>ESQPSVFQCKKCFQIVGDSNAWVISHREYLSFTLSDAVENSVRVEDTFKRSDDGLCVYSELSCTRCNEVIGKVYNSTPIYLDDIRDMYTFSMDKLQAYQLGNLEHHH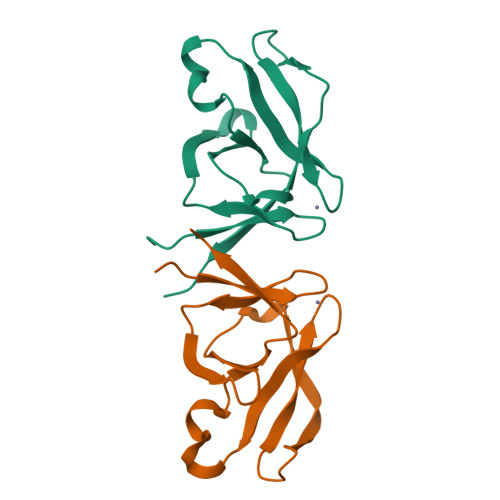HHH[3x]>MVQSLLEALNVRVVGSGE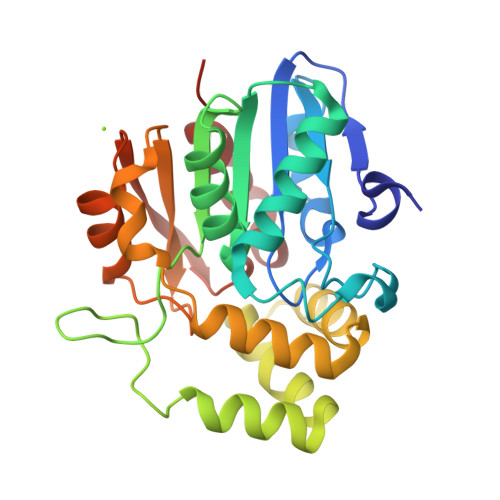KVLVLAHGVGTDQSAWQRILPYFVRDHRVVLYDLVCAGSVNPDYFDFRRYTSLDAFVDDLLAILDALRLGRCTYVGHSVSASIGILASIRRPDLFAKLILIGASPRFLNDKNYHGGFADGEIDTVFAAMEANYAAWVSGFAPLAVGADVPEAVREFSRTLFNMRPDITLFVSRMVFNSDLRGVLGLVTVPCSVLQTSKDHSVPESMAAYLKENLGGRTTVHMLDIEGHLPHLSAPNLLAQELRRALPR[2x]>MHHHHHHSSGRENLYFQGMPLRLDIKRKLTARSDRVKSVDLHPTEPWMLASLYNGSVCVWNHETQTLVKTFEVCDLPVRAAKFVARKNWVVTGADDMQIRVFNYNTLERVHMFEAHSDYIRCIAVHPTQPFILTSSDDMLIKLWDWDKKWSCSQVFEGHTHYVMQIVINPKDNNQFASASLDRTIKVWQLGSSSPNFTLEGHEKGVNCIDYYSGGDKPYLISGADDRLVKIWDYQNKTCVQTLEGHAQNVSCASFHPELPIIITGSEDGTVRIWHSSTYRLESTLNYGMERVWCVASLRGSNNVALGYDEGSIIVKLGREEPAMSMDANGKIIWAKHSEVQQANLKAMGDAEIKDGERLPLAVKDMGSCEIYPQTIQHNPNGRFVVVCGDGEYIIYTAMALRNKSFGSAQEFAWAHDSSEY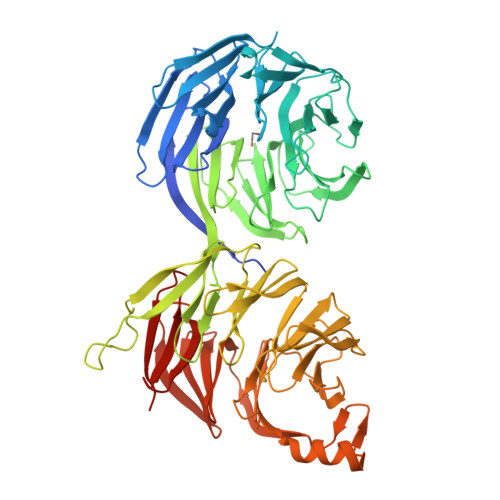AIRESNSIVKIFKNFKEKKSFKPDFGAESIYGGFLLGVRSVNGLAFYDWDNTELIRRIEIQPKHIFWSDSGELVCIATEESFFILKYLSEKVLAAQETHEGVTEDGIEDAFEVLGEIQEIVKTGLWVGDCFIYTSSVNRLNYYVGGEIVTIAHLDRTMYLLGYIPKDNRLYLGDKELNIISYSLLVSVLEYQTA[2x]> GADLADRFAELERRYDARLGVYVPATGTTAAIEYRADERFAFCSTFKAPLVAAVLHQNPLTHLDKLITYTSDDIRSISPVAQQHVQTGMTIGQLCDAAIRYSDGTAANLLLADLGGPGGGTAAFTGYLRSLGDTVSRLDAEEPELNRDPPGDERDTTTPHAIALVLQQLVLGNALPPDKRALLTDWMARNTTGAKRIRAGFPADWKVIDKTGTGDYGRANDIAVVWSPTGVPYVVAVMSDR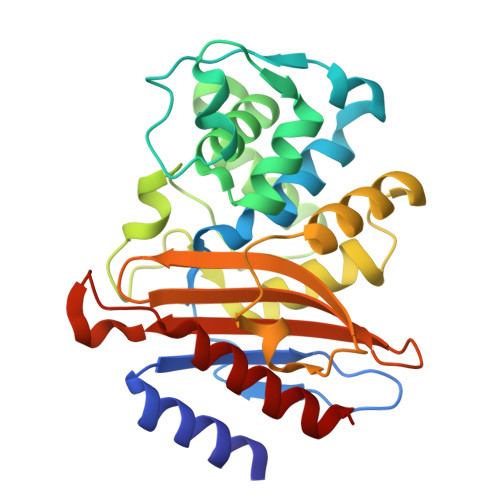AGGGYDAEPREALLAEAATCVAGVLA> MERYENLFAQLNDRREGAFVPFVTLGDPGIEQSLKIIDTLIDAGADALELGVPFSDPLADGPTIQNANLRAFAAGVTPAQCFEMLALIREKHPTIPIGLLMYANLVFNNGIDAFYARCEQVGVDSVLVADVPVEESAPFRQAALRHNIAPIFICPPNADDDLLRQVASYGRGYTYLLSRSGVTGAENRGALPLHHLIEKLKEYHAAPALQGFGISSPEQVSAAVRAGAAGAISGSAIVKI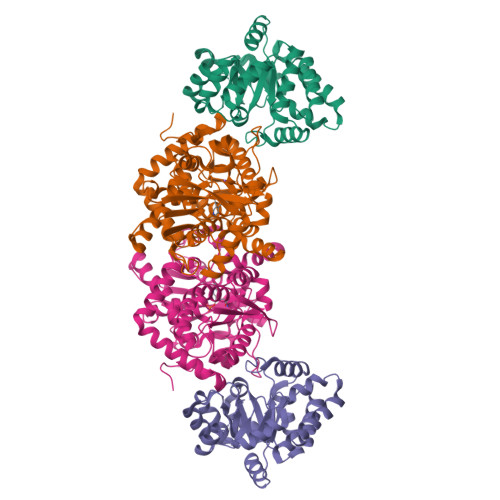IEKNLASPKQMLAELRSFVSAMKAASRA;> MTTLLNPYFGEFGGMYVPQILMPALNQLEEAFVSAQKDPEFQAQFADLLKNYAGRPTALTKCQNITAGTRTTLYLKREDLLHGGAHKTNQVLGQALLAKRMGKSEIIAETGAGNHGVASALASALLGLKCRIYMGAKDVERQSPNVFRMRLMGAEVIPVHSGSATLKDACNEALRDWSGSYETAHYMLGTAAGPHPYPTIVREFQRMIGEETKAQILDKEGRLPDAVIACVGGGSNAIGMFADFINDTSVGLIGVEPGGHGIETGEHGAPLKHGRVGIYFGMKAPMMQTADGQIEESYSISAGLDFPSVGPQHAYLNSIGRADYVSITDDEALEAFKTLCRHEGIIPALESSHALAHALKMMREQPEKEQLLVVNLSGRGDKDIFTVHDILKARGEI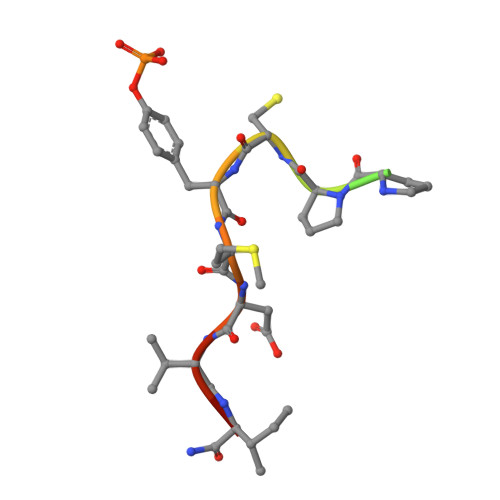> XTPEAPPCYMDVIX> KRHRKV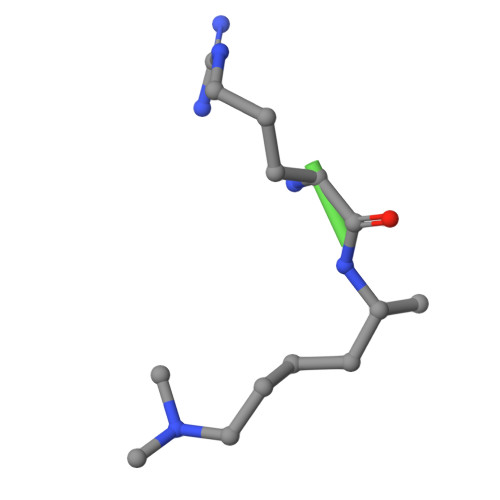LRDN> MTGMSREEVESLIQEVLEVYPEKARKDRNKHLAVNDPAVTQSKKCIISNKKSQPGLMTIRGCAYAGSKGVVWGPIKDMIHISHGPVGCGQYSRAGRRNYYIGTTGVNAFVTMNFTSDFQEKDIVFGGDKKLAKLIDEVETLFPLNKGISVQSECP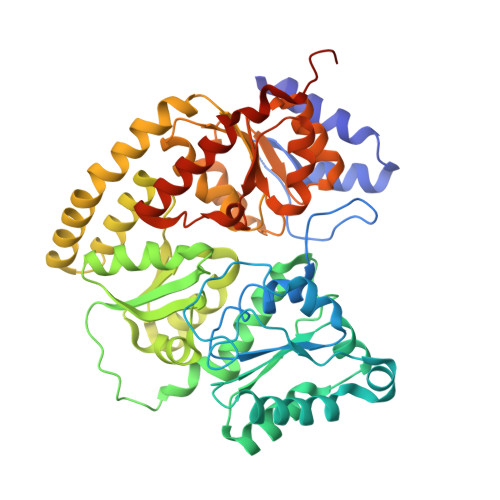IGLIGDDIESVSKVKGAELSKTIVPVRCEGFRGVSQSLGQHIANDAVRDWVLGKRDEDTTFASTPYDVAIIGDYNIGGDAWSSRILLEEMGLRCVAQWSGDGSISEIELTPKVKLNLVHCYRSMNYISRHMEEKYGIPWMEYNFFGPTKTIESLRAIAAKFDESIQKKCEEVIAKYKPEWEAVVAKYRPRLEGKRVMLYIGGLRPRHVIGAYEDLGMEVVGTGYEFAHNDDYDRTMKEMGDSTLLYDDVTGYEFEEFVKRIKPDLIGSGIKEKFIFQKMGIPFREMHSWDYSGPYHGFDGFAIFARDMDMTLNNPCWKKLQAPWEASEGAEKVAASA> GPYASLTEIEHLVQSVCKSYRETCQLRLEDLLRQRSNIFSREEVTGYQRKSMWEMWERCAHHLTEAIQYVVEFAKRLSGFMELCQNDQIVLLKAGAMEVVLVR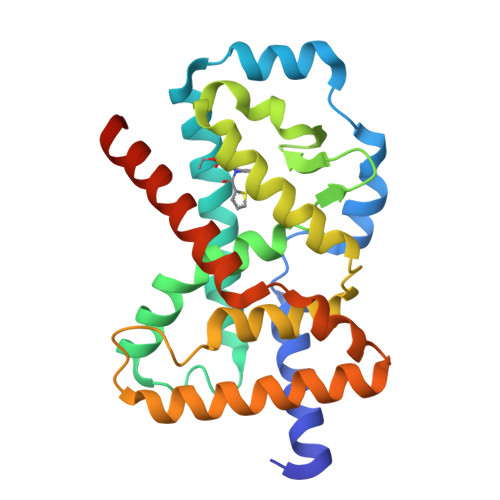MCRAYNADNRTVFFEGKYGGMELFRALGCSELISSIFDFSHSLSALHFSEDEIALYTALVLINAHRPGLQEKRKVEQLQYNLELAFHHHLSKTHRQSILAKLPPKGKLRSLCSQHVERLQIFQHLHPIVVQAAFP> MRGSAMASINDSKILSLQNKKNALVDTSGYNAEVRVGDNVQLNTIYTNDFKLSSSGDKIIVNLNNNILYSAIYENSSVSFWIKISKDLTNSHNEYTIINSIEQNSGWKLCIRNGNIEWILQDVNRKYKSLIFDYSESLSHTGYTNKWFFVTITNNIMGYMKLYINGELKQSQKIEDLDEVKLDKTIVFGIDENIDENQMLWIRDFNIFSKELSNEDINIVYEGQILRNVIKDYWGNPLKFDTEYYIINDNYIDRYIAPESNVLVLVQYPDRSKLYTGNPITIK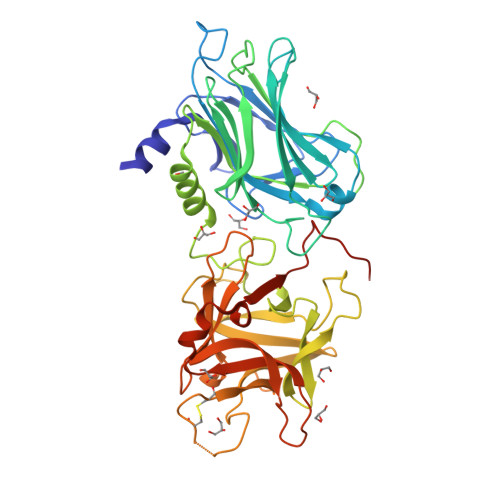SVSDKNPYSRILNGDNIILHMLYNSRKYMIIRDTDTIYATQGGECSQNCVYALKLQSNLGNYGIGIFSIKNIVSKNKYCSQIFSSFRENTMLLADIYKPWRFSFKNAYTPVAVTNYETKLLSTSSFWKFISRDPGWVEPPTPGWSHPQFEK Transfer RNA–guanine transglycosylase (Tgt, EC 2.4.2.29) catalyses the exchange of a specific guanine base in tRNA molecules by a substituted 7-deazaguanine. Bacterial Tgt functions as a homodimer in which the protomer consists of a (βα)8 barrel harbouring a Zn2+ binding subdomain close to the C-terminus. The reaction follows a ping-pong mechanism including a covalent Tgt⋅tRNA intermediate. Hence, in an attempt to generate a model system for the active site of human Tgt and to gain insights into the relevance of particular amino acids for substrate base selectivity, we adapted the Z. mobilis Tgt active site by site-directed mutagenesis in order to mimic that of the human enzyme.

Also the electron density maps of the Tgt(Val233Gly)·queuine and Tgt(Cys158Val/Val233Gly)·queuine complex structures enabled reliable placement of the 7-deazaguanine scaffold of the ligand which is, in both cases, similarly bound as in the Tgt(Cys158Val)·queuine complex. In both maps fragmentary density is visible for the dihydroxy-cyclopentenyl substituent (7H as well as 8F, 8H). Figures 7F and 7H show that the mutation of Val233 to glycine results in a considerable gain of space in the substrate binding pocket which allows the dihydroxy-cyclopentenyl of queuine to occupy the cavity located between Gly233 and the side chain of Cys/Val158. Within this cavity the dihydroxy-cyclopentenyl apparently has no specific interaction with the protein. As a consequence, it seems to be highly flexible which is reflected by the ill-defined electron density assigned to this moiety in both structures. The crystal structures of Tgt(Val233Gly) and Tgt(Cys158Val/Val233Gly) with queuine reveal that the Val233Gly exchange allows the dihydroxy-cyclopentenyl substituent to occupy the created cavity between position 233 and 158. The adopted binding mode of queuine will not interfere sterically with the sugar-phosphate backbone of bound tRNA. Yet, the results of the trapping experiment suggest that Tgt(Val233Gly) is also not able to bind queuine after the formation of the covalent enzyme·tRNA complex. It must be noted that in the case of all queuine complex structures determined in this study the electron density assigned to the 7-deazaguanine scaffold of the ligand by far does not comply with the nominal resolution of the respective structure. Even in the case of the mutated variants where reliable placement of the scaffold into the binding pocket was possible the electron density within this area appears rather fuzzy or even patchy and lacks detail. It is likely that multiple conformations and the low occupancy (on average 60%) of queuine in the binding pocket provoked the poor electron density.

> VEATAQETDRPRFSFSIAAREGKARTGTIEMKRGVIRTPAFMPVGTAATVKALKPETVRATGADIILGNTYHLMLRPGAERIAKLGGLHSFMGWDRPILTDSGGFQVMSLSSLTKQSEEGVTFKSHLDGSRHMLSPERSIEIQHLLGSDIVMAFDECTPYPATPSRAASSMERSMRWAKRSRDAFDSRKEQAENAALFGIQQGSVFENLRQQSADALAEIGFDGYAVGGLAGGEGQDEMFRVLDFSVPMLPDDKPHYLMGVGKPDDIVGAVERGIDMFDCVLPTRSGRNGQAFTWDGPINIRNARFSEDLKPLDSECHCAVCQKWSRAYIHHLIRAGEILGAMLMTEHNIAFYQQLMQKIRDSISEGRFSQFAQDFRARYFARNS>[6x]ENTLTVKMNDALSSGTGENIGEITVSETPYGLLFTPHLNGLTPGIHGFHVHTNPSCMPGMKDGKEVPALMAGGHLDPEKTGK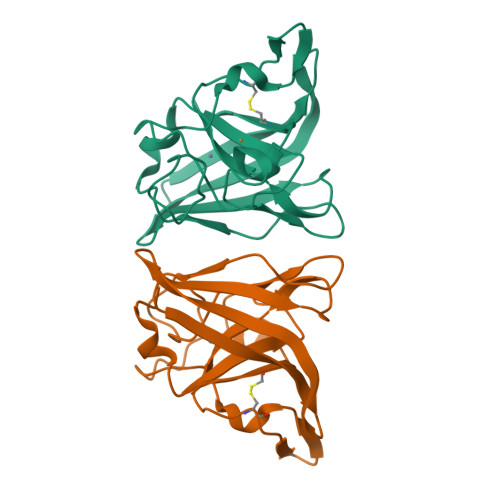HLGPYNDKGHLGDLPGLVVNADGTATYPLLAPRLKSLSELKGHSLMIHKGGDNYSDKPAPLGGGGARFACGVIEKLEHHHHHH> MTNESILESYSGVTPERKKSRMPAKLDWWQSATGLFLGLFMIGHMFFVSTILLGDNVMLWVT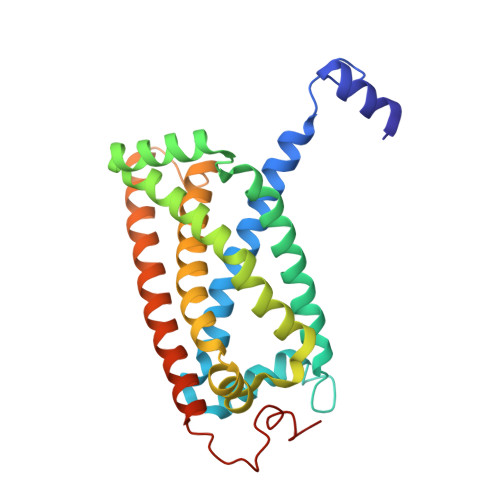KKFELDFIFEGGKPIVVSFLAAFVFAVFIAHAFLAMRKFPINYRQYLTFKTHKDLMRHGDTTLWWIQAMTGFAMFFLGSVHLYIMMTQPQTIGPVSSSFRMVSEWMWPLYLVLLFAVILHGSVGLYRLAVKWGWFDGETPDKTRANLKKLKTLMSAFLIVLGLLTFGAYVKKGLEQTDPNIDYKYFDYKRTHHR U-58872, HYDROXY DERIVATIVE 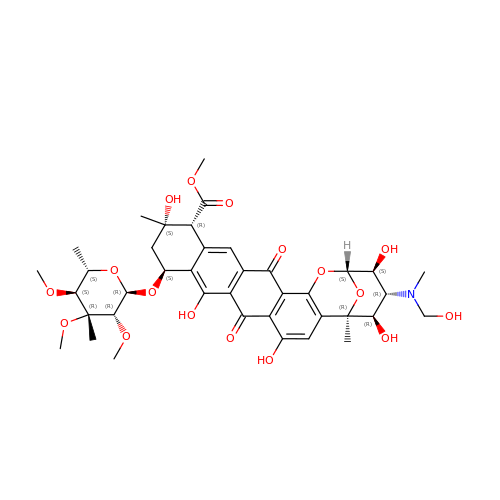OF NOGALAMYCIN | C39 H49 N O17 | LZNCBRPUGPTNSO-JYOBTZKQSA-N>[4x]MAAIAFIGLGQMGSPMASNLLQQGHQLRVFD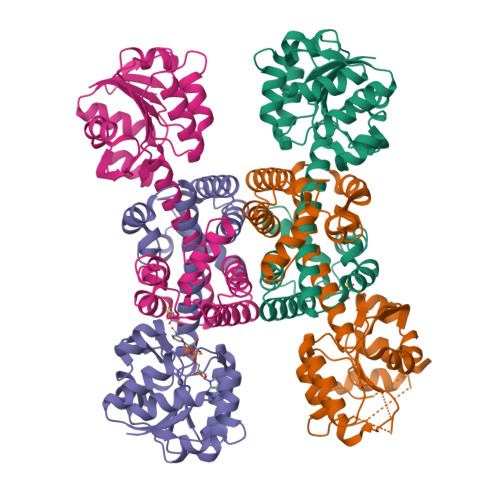VNAEAVRHLVDKGATPAANPAQAAKDAEFIITMLPNGDLVRNVLFGENGVCEGLSTDALVIDMSTIHPLQTDKLIADMQAKGFSMMDVPVGRTSANAITGTLLLLAGGTAEQVERATPILMAMGSELINAGGPGMGIRVKLINNYMSIALNALSAEAAVLCEALNLPFDVAVKVMSGTAAGKGHFTTSWPNKVLSGDLSPAFMIDLAHKDLGIALDVANQLHVPMPLGAASREVYSQARAAGRGRQDWSAILEQVRVSAGMTAKVKMLEHHHHHH> AFYKREMFDPAEKYKMDHRRRGIALIFNH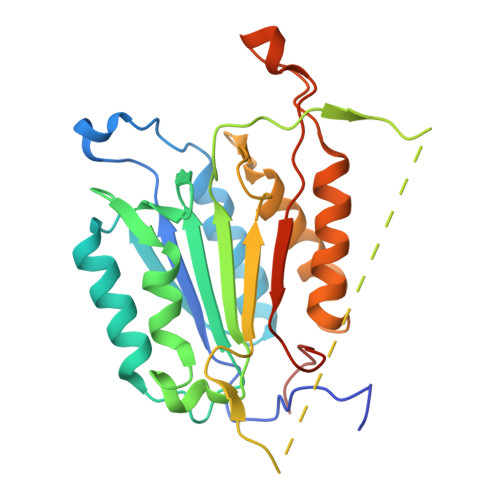ERFFWHLTLPERRGTCADRDNLTRRFSDLGFEVKCFNDLKAEELLLKIHEVSTVSHADADCFVCVFLSHGEGNHIYAYDAKIEIQTLTGLFKGDKCHSLVGKPKIFIIQACRGNQHDVPVIPLDVVDNQTEKLDTNITEVDAASVYTLPAGADFLMCYSVAEGYYSHRETVNGSWYIQDLCEMLGKYGSSLEFTELLTLVNRKVSQRRVDFCKDPSAIGKKQVPCFASMLTKKLHFFPKSNLEHHHHHH> MLSEAEEPREVATDVFNSKNLAVQAQKKILGKMVSKSIATTLIDDTSSEV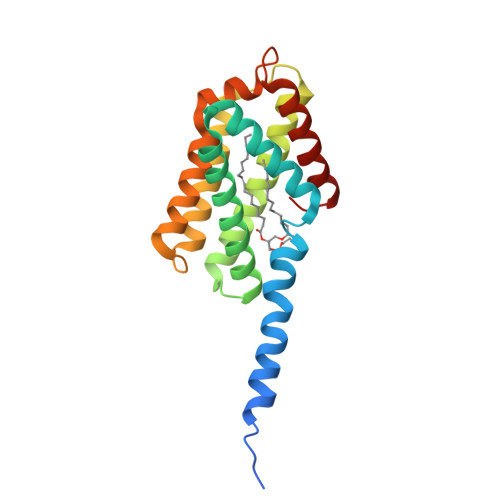LDELYRVTKEYTQNKKEAERVIKNLIKTVIKLAVLHRNNQFNQDELALMEKFKKKVHQLAMTVVSFHQVEYTFDRNVLSRLLNECRELLHEIIQRHLTAKSHGRVNNVFDHFSDSDFLAALYNPFGKFKPHLQKLCDGINKMLDEENI> MMYIQVLGSAAGGGFPQWNCNCVNCKGYRDGTLKATARTQSSIALSDDGVHWILCNASPDIRAQLQAFAPMQPARALRDTGINAIVLLDSQIDHTTGLLSLREGCPHQVWCTDMVHQDLTTGFPLFNMLSHWNGGLQWNRIELEGSFVIDACPNLKFTPFPLRSAAPPYSPHRFDPHPGDNLGLMVEDTRTGGKLFYAPGLGQVDEKLLA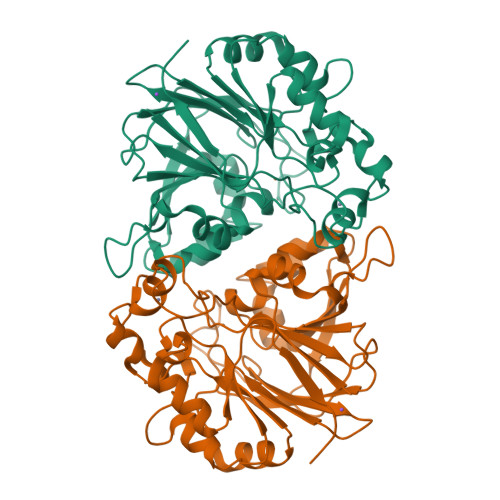MMHGADCLLVDGTLWEDDEMQRRGVGTRTGREMGHLAQNGPGGTLEVLDGFPRQRKVLIHINNTNPILDENSPERAEVLRRGVEVAFDGMSIELLEHH> FSLGLQDFDLLRVIGRGSYAKVLLVRLKKTDRIYAMKVVKKELVNDDEDIDWVQTEKHVFEQASNHPFLVGLHSCFQTESRLFFVIEYVNGGDLMFHMQRQRKLPEEHARFYSAEISLALNYLHERGIIYRDLKLDNVLLDSEGHIKLTDYGMCKEGLRPGDTTSTFCGTPNYIAPEILRGEDYGFSVDWWALGVLMFEMMAGRSPFDIVGSSDNPDQNTEDYLFQVILEKQIRIPRSLSVKAASVLKSFLNKDPKERLGCHPQTGFADIQGHPFFRNVDWDMMEQKQVVPPFKPNISGEFGLDNFDSQFTNEPVQLT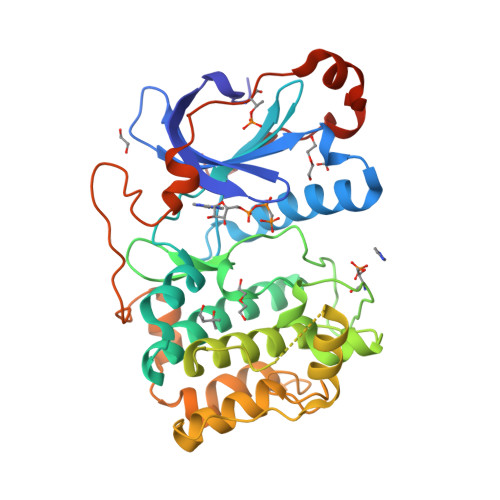PDDDDIVRKIDQSEFEGFEYINPLLMSAEECV> MDPQTLITKANKVSYYGNPTSKESWRYDWYQPSKVSSNVQQPQQQLGDMENNLEKYPFRYKTWLRNQEDEKNLQRESCEDILDLKEFDRRILKKSLMTSHTKGDTSKATG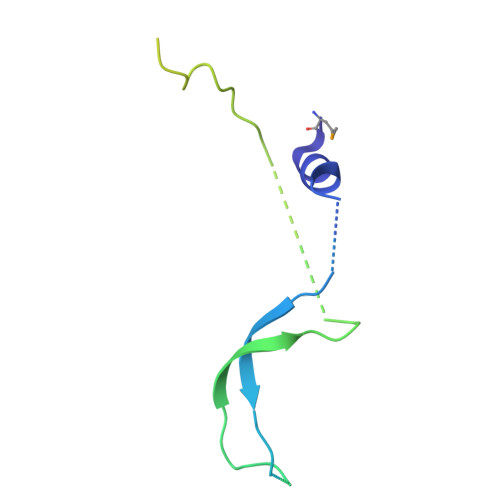APSANQGDEALSVDDIRGAVGNSEAIPGLSAGVNNDNTKESKDVKMN>[2x]MRGSHHHHHHGSMQILLANPRGFCAGVDRAISIVENALAIYGAPIYVRHEVVHNRYVVDSLRERGAIFIEQISEVPDGAILIFSAHGVSQAVRNEAKSRDLTVFDATCPLVTKVHMEVARASRRGEESILIGHAGHPDVEGTMGQYSNPEG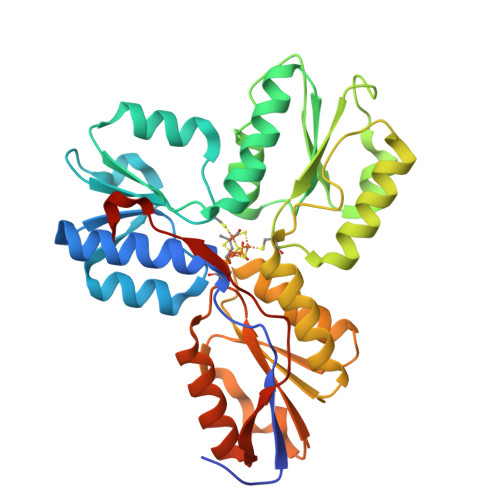GMYLVESPDDVWKLTVKNEEKLSFMTQTTLSVDDTSDVIDALRKRFPKIVGPRKDDICYATTNRQEAVRALAEQAEVVLVVGSKNSSNSNRLAELAQRMGKRAFLIDDAKDIQEEWVKEVKCVGVTAGASAPDILVQNVVARLQQLGGGEAIPLEGREENIVFEVPKELRVDIREVD>[2x]AKVGFIGAGKIGQTIAYSALVSGAVDEAVIYDIIPELPDKFEHELRHAFATKGIKANVLGTNSLDDVSGMDIVVISAGKPRKPGMSRRDLFVDNAKIMIDLAQKLPSKNPGAIYLMVANPVDMMASVFMKYSKQFTISAGDQVETMRMRSFIAKKLKIPVTSVDGFVGGEHGEDAVVLWSTVKIKGKPVDEFNINKDEVSDYVKKIPGEIIRVIGGTTWGPGTIIADIIK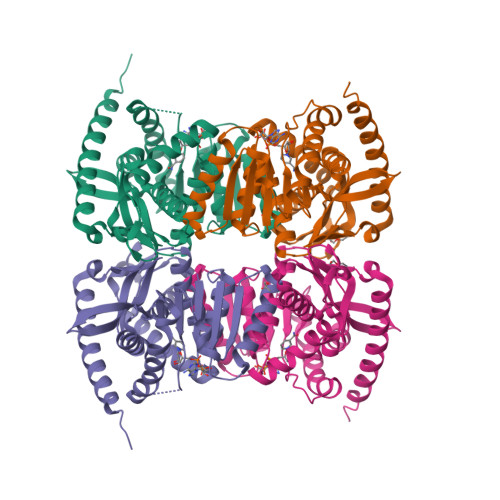SIAFSENRVMSIATPKEYEKEIIHVSAPTVVGSSIGPSLESLLDEKDRWHLNSAMKDFYEAYKENLKQLEQATKA> SECGPLQRLKVKRQWAEAYGSGNGREEFG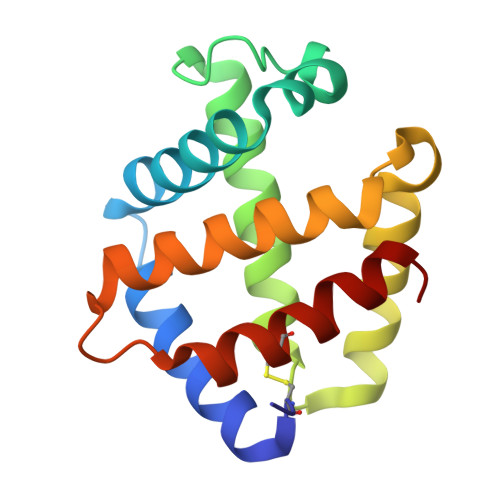HFIWANVFKVAPSARDMFKRVRGDNIYTPAFRAHATRVLGGLDMCVALLDDESVLNTQLAHLASQHSSRGVSAEQYNVVEHAVMMGVEHEIGQNVFDKDAWQACLDVITSGIQGN> GSGSAATDKFKAERATADTSPERLAAIAKDALGALNDVILKHGVTYPEYRVFKQWLIDVGEGGEWPLFLDVFIEHSVEEVLARSRKGTMGSIEGPYYIENSPELPSKCTLPMREEDEKITPLVFSGQVTDLDGNGLAGAKVELWHADNDGYYSQFAPHLPEWNLRGTIIADEEG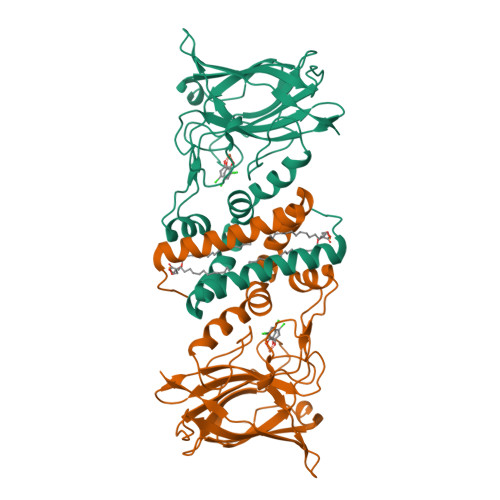RYEITTIQPAPYQIPTDGPTGQFIEAQNGHPWRPAHLHLIVSAPGKESVTTQLYFKGGEWIDSDVASATKPELILDPKTGDDGKNYVTYNFVLDPA> MSYPGKDKNIPGRIIEALEDLPLSYLVPKDGLAALVNAPMRVSLPFDKTIFTSADDGRDVNINVLGTANSTTSSIKNEAEKERLVFKRPSNFTSSANSVDYVPTNFLEGLSPLAQSVLSTHKGLNDSINIEKKSEIVSRPEAKHKLESVTSNAGNLSFNDNSSNKKTKTSTGVTMTQANLAEQYLNDLKNILDIVGFDQNSAEIGNIEYWLQLPNKKFVLTTNCLTKLQMTIKNITDNPQLSNSIEITWLLRLLDVMVCNIKFSKSSLKMGLDDSMLRYIALLSTIVLFNIFLLGKNDSNLHRESYIMEPVNFLSDLIESLKILTIEYGSLKIEFDTFQEALELLPKYIRNGPFLDDNVTAKLVYIFSDLLMNNDIEATTNIQFQSFWDNVKRISSDILVSLFGSFDQQRGFIIEELLSHIEKLPTKRIQKKLRKVGNQNIYITDFTFTLMSMLENINCYSFCNQMKDIAPENIDLLKNEYKKQEEFLFNIVEHINDTILERFFKNPSALRYVIDNFVQDLLLLISSPQWPVTEKILSSLLKRLLSVYSPSMQVSANIETICLQLIGNIGSTIFDIKCSTRDHEDNNLIKMINYPETLPHFFKSFEECIAYNETIKCRRSATRFLWNLRLGTILILEEYTKDAKEQIITVDNELKKILEQIKDGGLGPELENREADFSTIKLDYFSILHAFELLNLYDPYLKLILSLLAKDKIKLRSTAIKCLSMLASKDKVILSNPMVKETIHRRLNDSSASVKDAILDLVSINSSYFEFYQQINNNYNDDSIMVRKHVLRINEKMYDETNDIVTKVYVIARILMKIEDEEDNIIDMARLILLNRWILKVHEVLDQPEKLK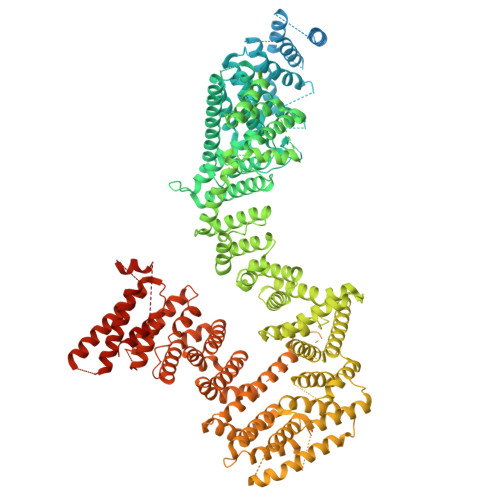EISSSVLLVMSRVAIMNEKCSQLFDLFLNFYLLNKEAHSKEAYDKITHVLTILTDFLVQKIVELNSDDTNEKNSIVDKQNFLNLLAKFADSTVSFLTKDHITALYPYMVSDEKSDFHYYILQVFRCTFEKLANFKQKFLYDLETTLLSRLPKMNVREIDEAMPLIWSVATHRHDTARVAKACSSCLSHLHPYINKANNEEAAIVVDGKLQRLIYLSTGFARFCFPKPSNDKIAFLQEGETLYEHITKCLLVLSKDKITHVIRRVAVKNLTKLCGNHPKLFNSRHVLHLLDKEFQSDQLDIKLVILESLYDLFLLEERKSVRNTGVNSTLSSNSILKKKLLKTNRVEFANDGVCSALATRFLDNILQLCLLRDLKNSLVAIRLLKLILKFGYTNPSHSIPTVIALFASTSQYIRHVAYELLEDLFEKYETLVFSSLSRGVTKAIHYSIHTDEKYYYKHDHFLSLLEKLCGTGKKNGPKFFKVLKRIMQSYLDDITDLTSTNSSVQKSIFVLCTNISNITFVSQYDLVSLLKTIDLTTDRLKEVIMDEIGDNVSSLSVSEEKLSGIILIQLSLQDLGTYLLHLYGLRDDVLLLDIVEESELKNKQLPAKKPDISKFSAQLENIEQYSSNGKLLTYFRKHVKDT> GPLGSVREEIESLVQDSLMEMVKGVKNTIESDLASKKGLAQSTTEILQLDPTNKAFAKS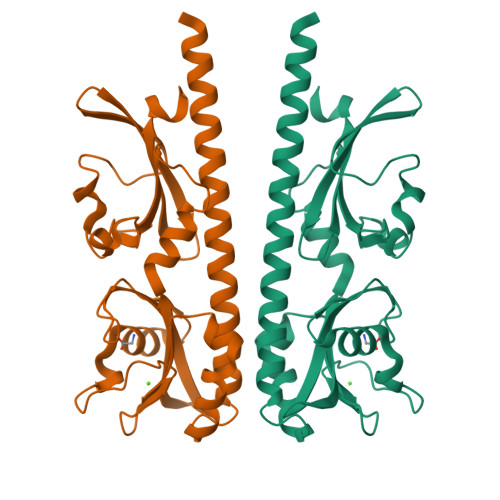VLESPNLKGSFLAIGLGYESDATVVENDDGWEPNADYDPRKRPWYVDAKRERKLVVTEPYVDISTKKIIISIGTPVYQQSNFVGAMFYDVELTQLAQLVNSVNLFDAGYLFITTKDGVTIAHPNAENNGEKFSQFLPNVDLKEGTQRIELDGKYYLVKFAQVPSESWYIGAVVDESIAFAMVDDLRHSSLIHHHHHH>MLKPDNLPVTFGKNDVEIIARETLYRGFFSLDLYRFRHRLFNGQMSHEVRREIFERGHAAVLLPFDPVRDEVVLIEQIRIAAYDTSETPWLLEMVAGMIEEGESVEDVARREAIEEAGLIVKRTKPVLSFLA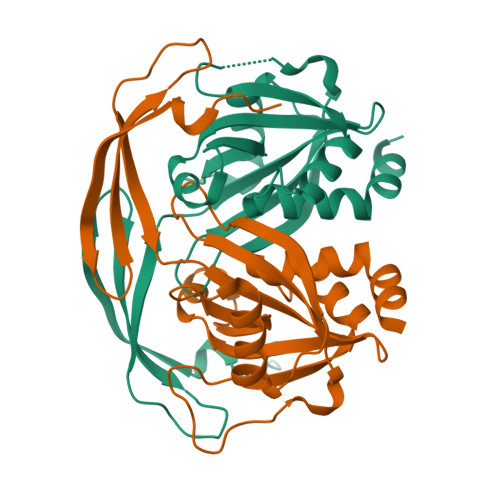SPGGTSERSSIMVGEVDATTASGIHGLADENEDIRVHVVSREQAYQWVEEGKIDNAASVIALQWLQLHHQALKNEWA[2x]2-[3-{4-chloro-3-[(4-chlorophenyl)ethynyl]phenyl}-1-(3-morpholin-4-ylpropyl)-1,4,6,7-tetrahydro-5H-pyrazolo[4,3-c]pyridin-5-yl]-2-oxoethanol 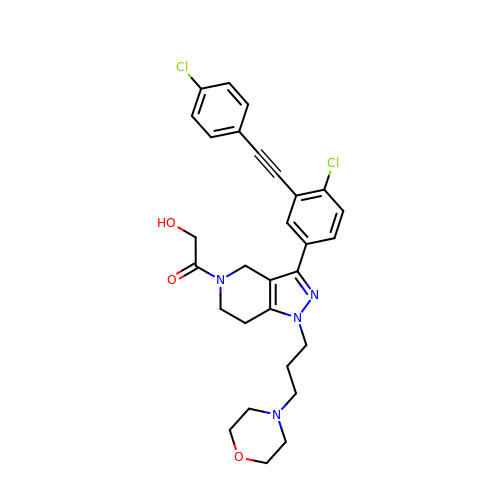| C29 H30 Cl2 N4 O3 | IWTCFPKHJADUJG-UHFFFAOYSA-N>[3x]KPVTLYDVAEYAGVSYQTVSRVVNQASHVSAKTREKVEAAMAELNYIPNRVAQQLAGKQLLLIGVATSSLALHAPSQIVAAIKSRADQLGASVVVSMVERSGVEACKAAVHNLLAQRVSGLIINYPLDDQDAIAVEAACTNVPALFLDVSDQTPINSIIFSHEDGTR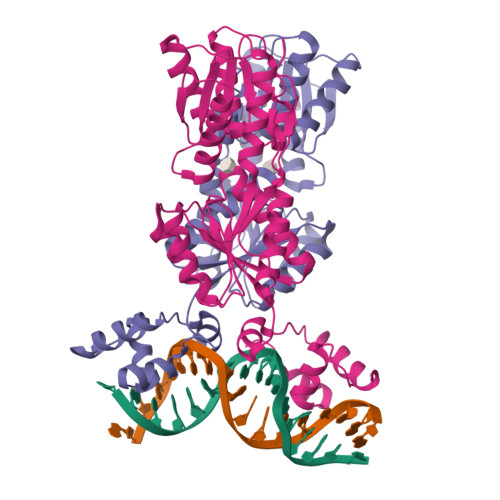LGVEHLVALGHQQIALLAGPLSSVSARLRLAGWHKYLTRNQIQPIAEREGDWSAMSGFQQTMQMLNEGIVPTAMLVANDQMALGAMRAITESGLRVGADISVVGYDDTEDSSCYIPPLTTIKQDFRLLGQTSVDRLLQLSQGQAVKGNQLLPVSLVKRKTTLA>MAAAAAEEGMEPRALQYEQTLMYGRYTQDLGAFAKEEAARIRLGGPEPWKGPPSSRAAPELLEYGRSRCARCRVCSVRCHKFLVSRVGEDWIFLVLLGLLMALVSWVMDYAIAACLQAQQWMSRGLNTSILLQYLAWVTYPVVLITFSAGFTQILAPQAVGSGIPEMKTILRGVVLKEYLTLKTFIAKVIGLTCALGSGMPLGKEGPFVHIASMCAALLSKFLSLFGGIYENESRNTEMLAAACAVGVGCCFAAPIGGVLFSIEVTSTFFAVRNYWRGFFAATFSAFIFRVLAVWNRDEETITALFKTRFRLDFPFDLQELPAFAVIGIASGFGGALFVYLNRKIVQVMRKQKTINRFLMRKRLLFPALVTLLISTLTFPPGFGQFMAGQLSQKETLVTLFDNRTWVRQGLVEELEPPSTSQAWNPPRANVFLTLVIFILMKFWMSALATTIPVPCGAFMPVFVIGAAFGRLVGESMAAWFPDGIHTDSSTYRIVPGGYAVVGAAALAGAVTHTVSTAVIVFELTGQIAHILPVMIAVILANA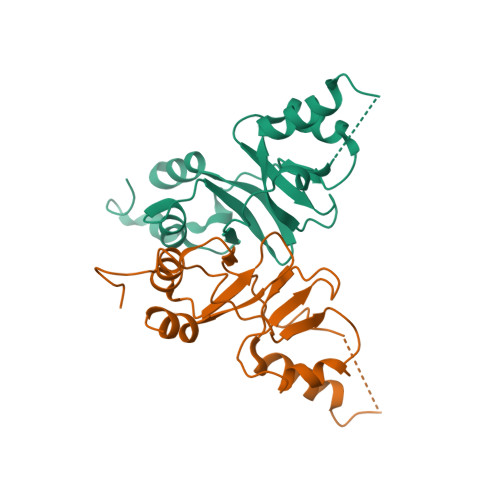VAQSLQPSLYDSIIRIKKLPYLPELGWGRHQQYRVRVEDIMVRDVPHVALSCTFRDLRLALHRTKGRMLALVESPESMILLGSIERSQVVALLGAQLSPARRRQHMQERRATQTSPLSDQEGPPTPEASVCFQVNTEDSAFPAARGETHKPLKPALKRGPSVTRNLGESPTGSAESAGIALRSLFCGSPPPEAASEKLESCEKRKLKRVRISLASDADLEGEMSPEEILEWEEQQLDEPVNFSDCKIDPAPFQLVERTSLHKTHTIFSLLGVDHAYVTSIGRLIGIVTLKELRKAIEGSVTAQGVKVRPPLASFRDSATSSSDTETTEVHALWGPHSRHGLPREGSPSDSDDKCQ[2x]>[2x]MIEITLKKPEDFLKVKETLTRMGIANNKDKVLYQSCHIL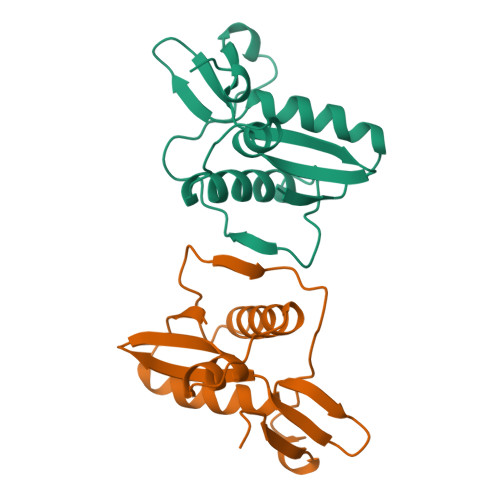QKKGLYYIVHFKEMLRMDGRQVEMTEEDEVRRDSIAWLLEDWGLIEIVPGQRTFMKDLTNNFRVISFKQKHEWKLVPKYTIGN>[2x]AHKAQQYYFDAAEAEAWMSEQELYMMSEEKAKDEQSAVSMLKKHQILEQAVEDYAETVHQLSKTSRALVADSHPESER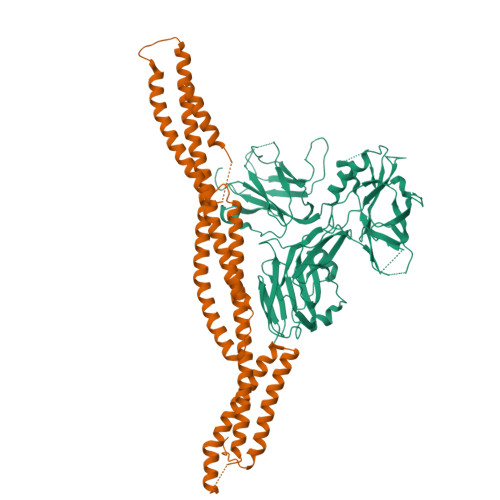ISMRQSKVDKLYAGLKDLAEERRGKLDERHRLFQLNREVDDLEQWIAEREVVAGSHELGQDYEHVTMLQERFREFARDTGNIGQERVDTVNNMADELINSGHSDAATIAEWKDGLNEAWADLLELIDTRTQILAASYELHKFYHDAKEIFGRIQDKHKKLPEELGRDQNTVETLQRMHTTFEHDIQALGTQVRQLQEDAARLQAAYAGDKADDIQKRENEVLEAWKSLLDACEGRRVRLVDT;>[2x]ADTLDNVNLVSSPVHSGFLVSFMVDARGGSMRGSRHHGMRIIIPPRKCTAPTRITCRLVKRHKLANPPPMVEGEGLASRLVEMGPAGAQFLGPVIVEIPHFGSMRGKERELIVLRSENGETWKEHQFDSKNEDLSELLNGMDEELDSPEELGTKRICRIITKDFPQYFAVVSRIKQESNQIGPEGGILSSTTVPLVQASFPEGALTKRIRVGLQAQPVPEETVKKILGNKATFSPIVTVEPRRRKFHKPITMTIPVPPPSGEGVSNGYKGDTTPSLRLLCSITGGTSPAQWEDITGTTPLTFIKDCVSFTTNVSARFWLADCHQVLETVGLASQLYRELICVPYMAKFVVFAKTNDPVESSLRCFCMTDDRVDKTLEQQENFEEVARSKDIEVLEGKPIYVDCYGNLAPLTKGGQQLVFNFYSFKENRLPFSIKVRDTSQEPCGRLSFLKEPKTTKGLPQTAVCNLNITLPAHKKAEKADRRQSFTSLALR> MITIDALGQVCPIPVIRAKKALAELGEAGGVVTVLVDNDISRQNLQKMAEGMGYQSEYLEKDNGVIEVTIVAGE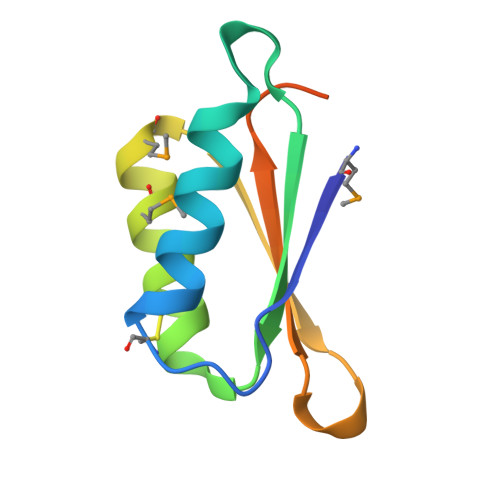GCAVELEHHHHHH> VEYKNTICPPRQDYRYWYFVAELTIGVNYDINSTIIGECHMSESYIDRNANIVLTGYGLKINMTIMDTDQRFVAAAEGVGKDNKLSVLLFTTQRLDKVHHNISVTITCMEMNCGTTKYNSDLPESIHKSSSCDITINGSCVTCVNLETDPTKINPHYLHPKNKYLYHNSEYSMRGSYGVTFIDE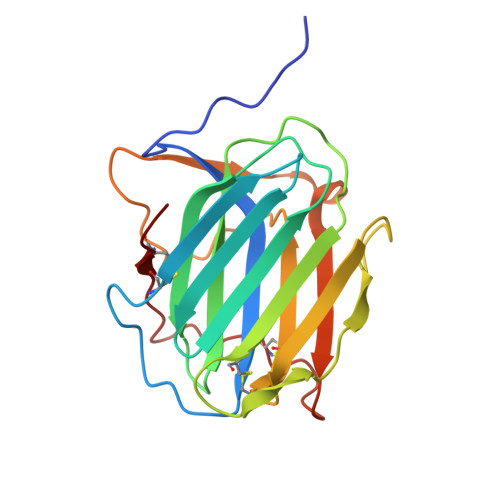LNQCLLDIKELSYDICYRE DIDECYL-DIMETHYL-AMMONIUM | C22 H48 N | 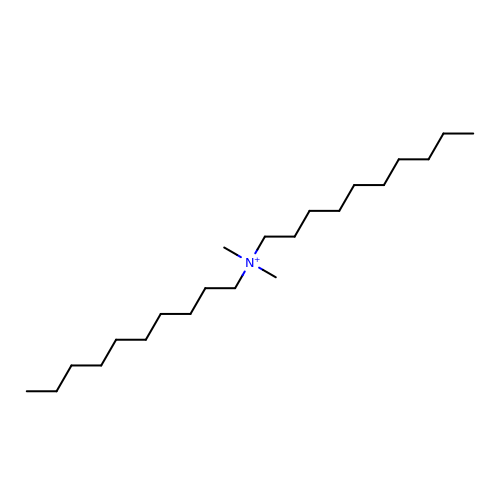JGFDZZLUDWMUQH-UHFFFAOYSA-N> GSHMEKRTPHTRLSQVKKLVNAG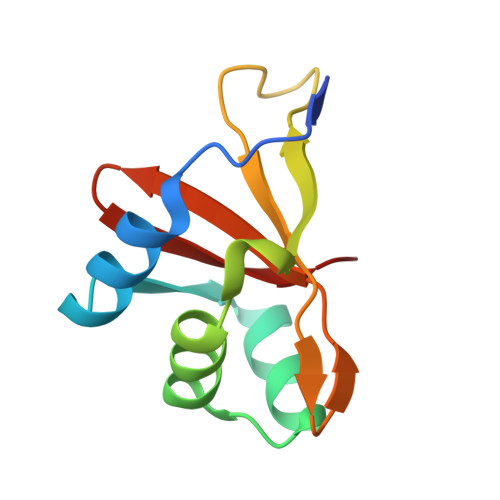QVRTTRSALLNADELGLDFDGMCNVIIGLSESDFYKSMTTYSDHTIWQDVYRPRLVTGQVYLKITVIHDVLIVSFKEK>MGPIPPTGVPVGDFFVCGRMTTLHMGGQSGIQATTLVNGMIYRTDHPEPSTSPVSNWEFTVLENNTIVGAGMGCVWFQKSEALVWTLDGQKLSGWNTLDGVGTTQLTVAWRQHNRTIYGWANVVAWNSEEWHTNAEQPHQPILRLTYWLVKINVLSEPEDFDVVQKSPLAYLEDYTTAQSKSAIQKLNFQTFQKPEGGGTLRAQYSTTPRQGDFAVIWQIGRHNFDMSTGKGTPVESLSDYVMPQQKDAHIGMWYRALTSVGPRTDVLTLHFHLPTVEKAAAELALVPR[2x]

The HAstV capsid precursor protein comprises several domains, including a highly basic amino terminus that binds to the RNA genome, a core domain that forms the icosahedral shell, a spike domain that forms dimeric protrusions, and an acidic domain with unknown function at the carboxy terminus. The HAstV-VA1 spike forms a dimer and shares a core beta-barrel structure with other astrovirus capsid spikes but is otherwise strikingly different, suggesting that HAstV-VA1 may utilize a different cell receptor, and an infection competition assay supports this hypothesis. The HAstV-VA1 spike structural domain forms a homodimer, with each protomer encompassing residues 408–684. Also similar to other HAstV spikes, the structural domain of each protomer of the HAstV-VA1 spike comprises a core antiparallel beta-barrel, formed by beta-strands 1, 9, 10, 16, and 18.

The HAstV-VA1neuro capsid spike structure provided a guide to generate a new construct encoding only the amino acids that form the HAstV-VA1 spike structural domain (residues 408–684), and this construct yielded a soluble protein in E. coli. We then used this strategy to generate a construct encoding the capsid spike structural domain from a gastrointestinal HAstV-VA1 (HAstV-VA1gastro) identified in 2008 in an individual with acute gastroenteritis. This recombinant HAstV-VA1gastro capsid spike protein forms a dimer in solution, consistent with other HAstV capsid spikes. The HAstV-VA1gastro capsid spike was then crystallized and its structure was solved to 1.46 Å resolution. Structural alignment of the experimentally-determined HAstV-VA1 spike crystal structure with the Alphafold2 predicted model using TM-align revealed an RMSD of 2.90 Å across 264 residue pairs and a TM-score of 0.85, revealing a relatively accurate match in the beta-strand and alpha-helical regions and significant differences in the loop regions. Finally, to evaluate if there are structural changes in the spike that drive infection of the CNS, we aligned the HAstV-VA1gastro and HAstV-VA1neuro spike structures, which resulted in an RMSD of 0.78 Å and TM-score of 0.97, revealing that no major structural differences are observed. We observed that the HAstV-VA1gastro spike sequence is generally more conserved than the HAstV-VA1neuro spike sequence. Specifically, only six variable sites were observed in HAstV-VA1gastro spike sequences, whereas 27 variable sites were observed in HAstV-VA1neuro spike sequences. Statistical analyses confirm that there is a significant decrease in antibody binding to the HAstV-VA1neuro spike compared to the HAstV-VA1gastro spike. While these results are not entirely surprising given that the antibodies were raised against a gastrointestinal HAstV-VA1 strain, they do demonstrate that antibodies to a gastrointestinal HAstV-VA1 virus are less reactive to neuronal HAstV-VA1 spike compared to gastrointestinal HAstV-VA1 spike.> ILPSFIEHSSFGVKESNPYNKLFEERIIFLGVQVDDASANDIMAQLLVLESLDPDRDITMYINSPGGGFTSLMAIYDTMQYV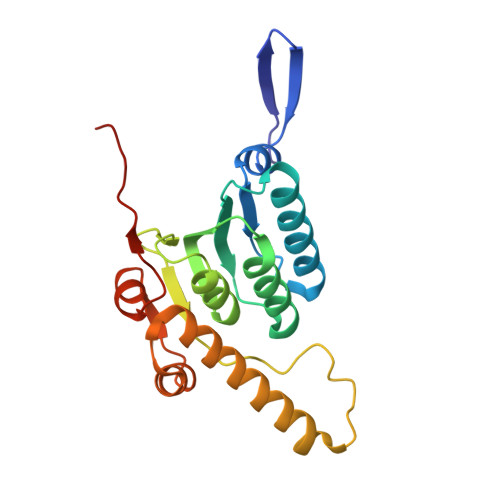RADIQTVCLGQAASAAAVLLAAGTPGKRMALPNARVLIHQPSLSGVIQGQFSDLEIQAAEIERMRTLMETTLARHTGKDAGVIRKDTDRDKILTAEEAKDYGIIDTVLEYRKLSAQTA>MSERLSITPLGPYIGAQISGADLTRPLSDNQFEQLYHAVLRHQVVFLRDQAITPQQQRALAQRFGELHIHPVYPHAEGVDEIIVLDTHNDNPPDNDNWHTDVTFIETPPAGAILAAKELPSTGGDTLWTSGIAAYEALSVPFRQLLSGLRAEHDFRKSFPEYKYRKTEEEHQRWREAVAKNPPLLHPVVRTHPVSGKQALFVNEGFTTRIVDVSEKESEALLSFLFAHITKPEFQVRWRWQPNDIAIWDNRVTQHYANADYLPQRRIMHRATILGDKPFYRAG[4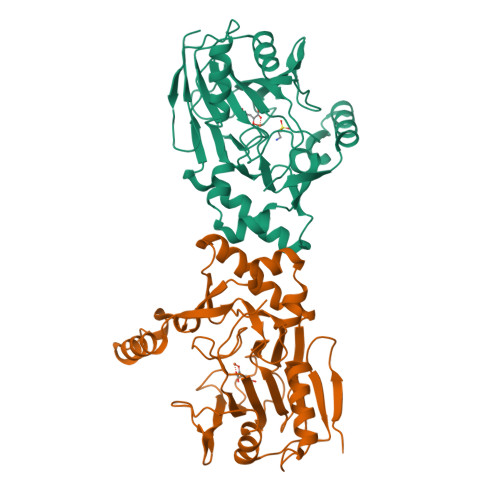x]> AIGEFMVSLPRMVYPQPKVLTPCRKDVLVVTPWLAPIVWEGTFNIDILNEQFRLQNTTIGLTVFAIKKYVAFLKLFLETAEKHFMVGHRVHYYVFTDQPAAVPRVTLGTGRQLSVLEVRAYKRWQDVSMRRMEMISDFCERRFLSEVDYLVCVDVDMEFRDHVGVEILTPLFGTLHPGFYGSSREAFTYERRPQSQAYIP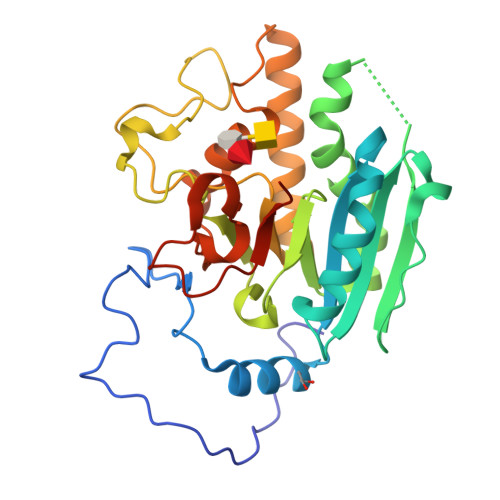KDEGDFYYLGGFFGGSVQEVQRLTRACHQAMMVDQANGIEAVWHDESHLNKYLLRHKPTKVLSPEYLWDQQLLGWPAVLRKLRFTAVPKNHQAVRNP> STDNAETGVIEAGNTDTDFSGELAAPGSNHTNVKFLFDRSRLLNVIKVLEKDAVFPRPFPTATGTQQDDGYFCLLTPRPTVASRPATRFGLYVSPSDSGVLANTSLDFNFYSLACFTYFRSDLEVTVVSLEPDLEFAVGWFPSGSEYQASSFVYDQLHVPYHFTGRTPRAFASKGGKVSFVLPWNSVSSVLPVRWGGASKLSSATRGLPAHADWGTIYAFIPRPNEKKSTAVKHVAVYIRYKNARAWCPSMLPFRSYK;> DRVTTQTAGNTAINTQSSLGVLCAYVEDPTKSDPPSSSTDQPTTTFTAIDRWYTGRLNSWTKAVKTFSFQAVPLPGAFLSRQGGLNGGAFTATLHRHFLMKCGWQVQVQCNLTQFHQGALLVAMVPETTLDVKPDGKAKSLQELNEEQWVEMSDDYRTGKNMPFQSLGTYYRPPNWTWGPNFINPYQVTVFPHQILNARTSTSVDINVPYIGETPTQSSETQNSWTLLVMVLVPLDYKEGATTDPEITFSVRPTSPYFNGLRNRYTT;> GPIPTAPRENSLMFLSTTPDDTVPAYGNVRTPPVNYLPGEITDLLQLARIPTLMAFGRVDAYVPYVAVPTQFDDKPLISFPITLSDPVYQNTLVGAISSNFANYRGCIQITLTFCGPMMARGKFLLSYSPPNGTQPQTLSEAMQCTYSIWDIGLNSSWTFVIPYISPSDYRE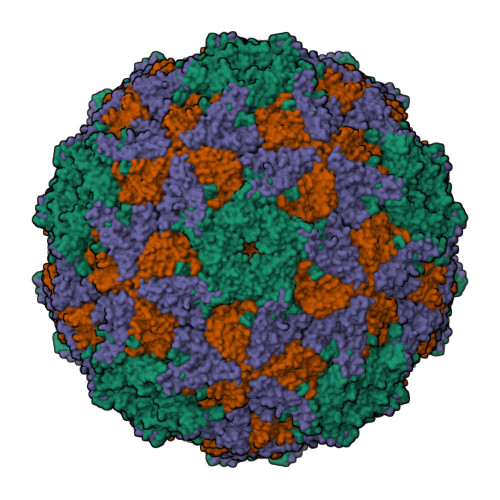TRAITNSVYSADGWFSLHKLTKITLPPDCPQSPCILFFASAGEDYTLRLPVDCNPSYVF;> GNVQTTSKNDFDSRGNNGNMTFNYYANTYQNSVDFSTSSSASGAGPGNSRGGLAGLLTNFSGILNPLGYLK>MRIPLVGKDSIESKDIGFTLIHEHLRVFSEAVRQQWPHLYNEDEEFRNAVNEVKRAMQFGVKTIVDPTVMGLGRDIRFMEKVVKATGINLVAGTGIYIYIDLPFYFLNRSIDEIADLFIHDIKEGIQGTLNKAGFVKIAADEPGITKDVEKVIRAAAIANKETKVPIITHSNAHNNTGLEQQRILTEEGVDPGKILIGHLGDTDNIDYIKKIADKGSFIGLDRYGLDLFLPVDKRNETTLRLIKDGYSDKIMISHDYCCTIDVGTAKPEYKPKLAPRWSITLIFEDT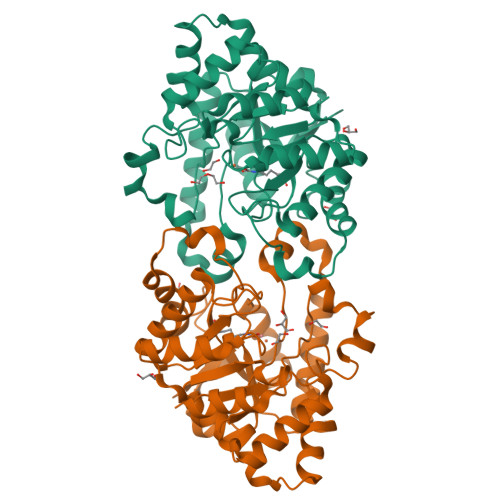IPFLKRNGVNEEVIATIFKENPKKFFS[4x]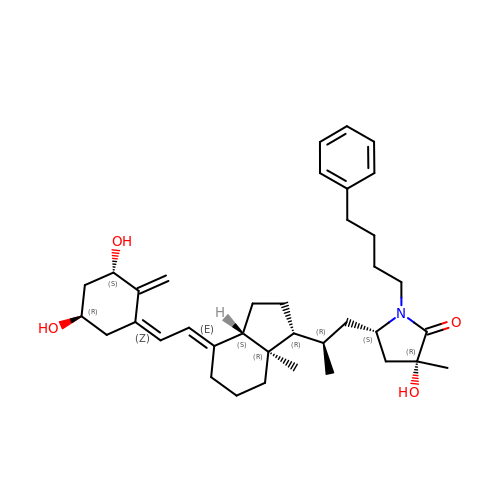(3R,5S)-5-[(2R)-2-[(1R,3aS,4E,7aR)-7a-methyl-4-[(2Z)-2-[(3S,5R)-2-methylidene-3,5-bis(oxidanyl)cyclohexylidene]ethylidene]-2,3,3a,5,6,7-hexahydro-1H-inden-1-yl]propyl]-3-methyl-3-oxidanyl-1-(4-phenylbutyl)pyrrolidin-2-one | C37 H53 N O4 | IVUJLUOFPHOBPG-HEMHZJQPSA-N>MAKRSLRKMWRPGEKKEPQGVVYEDVPDDTEDFKESLKVVFEGSAYGLQNFNKQKKLKRCDDMDTFFLHYAAAEGQIELMEKITRDSSLEVLHEMDDYGNTPLHCAVEKNQIESVKFLLSRGANPNLRNFNMMAPLHIAVQGMNNEVMKVLLEHRTIDVNLEGENGNTAVIIACTTNNSEALQILLKKGAKPCKSNKWGCFPIHQAAFSGSKECMEIILRFGEEHGYSRQLHINFMNNGKATPLHLAVQNGDLEMIKMCLDNGAQIDPVEKGRCTAIHFAATQGATEIVKLMISSYSGSVDIVNTTDGCHETMLHRASLFDHHELADYLISVGADINKIDSEGRSPLILATASASWNIVNLLLSKGAQVDIKDNFGRNFLHLTVQQPYGLKNLRPEFMQMQQIKELVMDEDND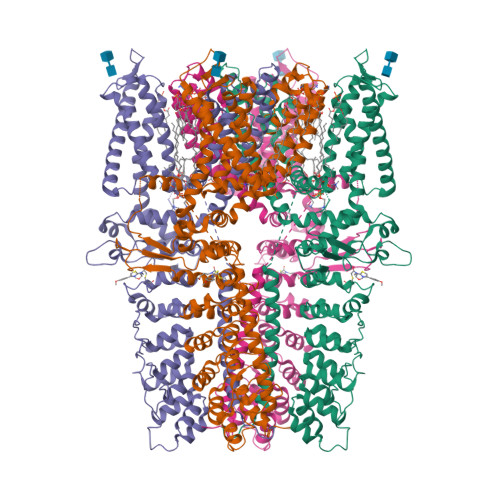GCTPLHYACRQGGPGSVNNLLGFNVSIHSKSKDKKSPLHFAASYGRINTCQRLLQDISDTRLLNEGDLHGMTPLHLAAKNGHDKVVQLLLKKGALFLSDHNGWTALHHASMGGYTQTMKVILDTNLKCTDRLDEDGNTALHFAAREGHAKAVALLLSHNADIVLNKQQASFLHLALHNKRKEVVLTIIRSKRWDECLKIFSHNSPGNKCPITEMIEYLPECMKVLLDFCMLHSTEDKSCRDYYIEYNFKYLQCPLEFTKKTPTQDVIYEPLTALNAMVQNNRIELLNHPVCKEYLLMKWLAYGFRAHMMNLGSYCLGLIPMTILVVNIKPGMAFNSTGIINETSDHSEILDTTNSYLIKTCMILVFLSSIFGYCKEAGQIFQQKRNYFMDISNVLEWIIYTTGIIFVLPLFVEIPAHLQWQCGAIAVYFYWMNFLLYLQRFENCGIFIVMLEVILKTLLRSTVVFIFLLLAFGLSFYILLNLQDPFSSPLLSIIQTFSMMLGDINYRESFLEPYLRNELAHPVLSFAQLVSFTIFVPIVLMNLLIGLAVGDIAEVQKHASLKRIAMQVELHTSLEKKLPLWFLRKVDQKSTIVYPNKPRSGGMLFHIFCFLFCTGEIRQEIPNADKSLEMEILKQKYRLKDLTFLLEKQHELIKLIIQKMEIISETEDDDSHCSFQDRFKKEQMEQRNSRWNTVLRAVKAKTHHLEPSNSLEVLFQGPAADYKDDDDKAHHHHHHHHHH[4x]> MLRDLFDRAVVLSHYIHNLSSEMFSEFDKRYTHGRGFITKAINSCHTSSLATPEDKEQAQQMNQKDFLSLIVSILRSWNEPLYHLVTEVRGMQEAPEAILSKAVEI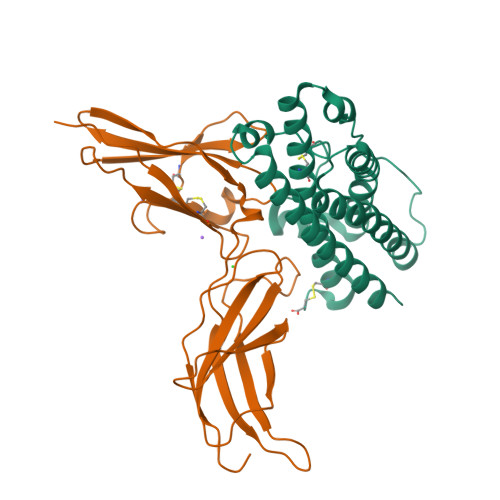EEQTKRLLERMELIVSQVHPETKENEIYPVWSGLPSLQMADEESRLSAYYNLLHCLRRDSHKIDNYLKLLKCRIIHNNNC;> MLPPGKPEIFKCRSPNKETFTCWWRPGTDGGLPTNYSLTYHREGETLMHECPDYITGGPNSCHFGKQYTSMWRTYIMMVNATNQMGSSFSDELYVDVTYIVQPDPPLELAVEVKQPEDRKPYLWIKWSPPTLIDLKTGWFTLLYEIRLKPEKAAEWEIHFAGQQTEFKILSLHPGQKYLVQVRCKPDHGYWSAWSPATFIQIPSDFTMND>[2x]ANNRAEVDTLSPAQAAELKPMPQSWRGVL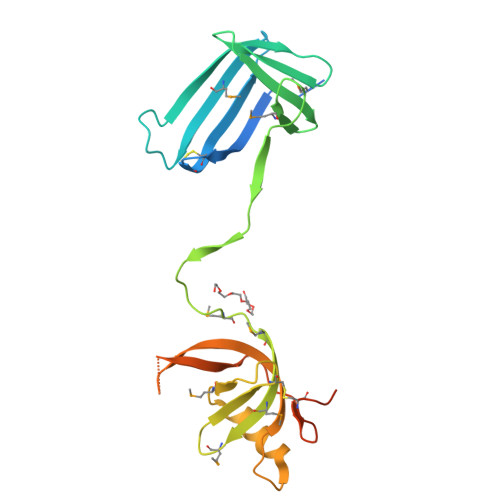PCADCEGIETSLFLEKDGTWVMNERYLGAREEPSSFASYGTWARTADKLVLTDSKGEKSYYRAKGDALEMLDREGNPIESQFNYTLEAAQSSLPMTPMTLRGMYFYMADAATFTDCATGKRFMVANNAELERSYLAARGHSEKPVLLSVEGHFTLEGNPDTGAPTKVLAPDTAGKFYPNQDCSSLGQMASMTGGQQMGHHHHHH>GAMASHKLLVTPPKALLKPLSIPNQLLLGPGPSNLPPRIMAAGGLQMIGSMSKDMYQIMDEIKEGIQYVFQTRNPLTLVISGSGHCALEAALVNVLEPGDSFLVGANGIWGQRAVDIGERIGARVHPMTKDPGGHYTLQEVEEGLAQHKPVLLFLTHGESSTGVLQPLDGFGELCHRYKCLLLVDSVAFLGGTPLYMDRQGIDILYSGSQKALNAPPGTSLISFSDKAKKKMYSRKTKPFSFYLDIKWLANFWGCDDQPRMYHHTIPVISLYSLRESLALIAEQGLENSWRQHREAAAYLHGRLQALGLQLFVKDPALRLPTVTTVAVPAGYDWRDIVSYVIDHFDIEIMGGLGPSTGKVLRIGLLGCNATRENVDRVTEALRAALQHCPKKKL[4x]

Human alanine:glyoxylate aminotransferase (AGT) is a Fold-type I pyridoxal 5′-phosphate (PLP)-dependent enzyme, which catalyses the conversion of L-alanine and glyoxylate to pyruvate and glycine in liver peroxisomes. The protein is a 86 kDa-homodimer and each subunit comprises a 21-residues long N-terminal extension that wraps over the surface of the neighboring subunit and is important for the attainment of the correct conformation of the holo-protein, a 260-residues large domain containing most of the active site and of the dimerization interface, and a 110-residues C-terminal domain containing regions involved in the recognition and binding to the Pex5p peroxisomal receptor. The AGT aminotransferase reaction follows a ping-pong bi–bi mechanism that relies on the formation of the external aldimine intermediate, in which the amino group of L-alanine replaces the ɛ-amino group of Lys209, the PLP-binding residue. Inherited mutations of the AGXT gene lead to the rare metabolic disorder Primary Hyperoxaluria Type I (PH1) (MIM #259900).5 In the absence of functional AGT, glyoxylate is converted to oxalate by cytosolic lactate dehydrogenase (LDH).

Ser187 is a large-domain residue conserved in the mammalian AGTs and belongs to a random-coil region that is not part of the active site. In order to have a deeper understanding of the structural and functional effects of the S187F mutation on AGT, we have solved the X-ray crystal structure of the S187F variant to a resolution of 2.9 Å. The S187F structure superimposes well onto the normal AGT counterpart, with a root-mean-square deviation of 0.48 Å. Although the overall conformation of the two proteins is virtually identical, significant structural changes can be observed near the mutated amino acid as well as at the active site of the protein. As a result of the mutation, the loop that contains Phe187 substantially changes its conformation, and moves Phe187 into the position of Leu188 of normal AGT. Because of this displacement, the Val185 residue of the mutant protein also changes position, and its side chain moves away from the PLP. The small hydrophobic pocket that is formed by Phe187 and Leu188 can accommodate Ala210, which eventually causes a shift of Ala210 and Lys209 towards Phe187. In fact, the distance between the Cα of Lys209 and the C3 of the PLP methylpyridine ring decreases from 8.0 Å in the normal AGT enzyme to 6.5 Å in the mutant enzyme, and the distance between the Cα of Val185 and the C3 of the PLP methylpyridine ring increases from 4.9 Å in the normal AGT enzyme to 6.7 Å in the mutant. Moreover, as calculated by Pocket Finder, in S187F the PLP cavity has a volume of 1073 Å3, while in normal AGT it has a volume of 949 Å3.HYDROCINNAMIC ACID | C9 H10 O2 | 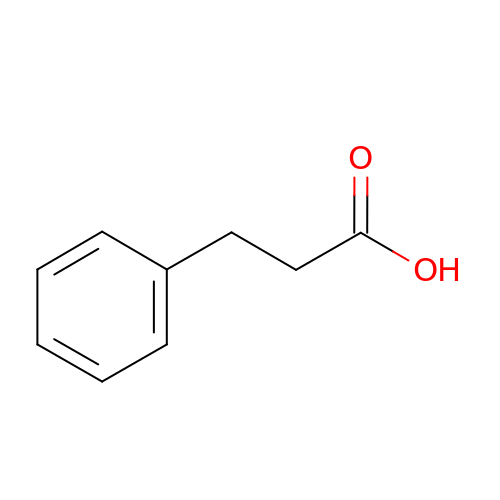XMIIGOLPHOKFCH-UHFFFAOYSA-N> MRLRSPYWLFVVLILALAGLQYRLWVGDGSLAQVRDLQKQIADQHGENERLLERNRILEAEVAELKKGTETVEERARHELGMVKDGETLYQL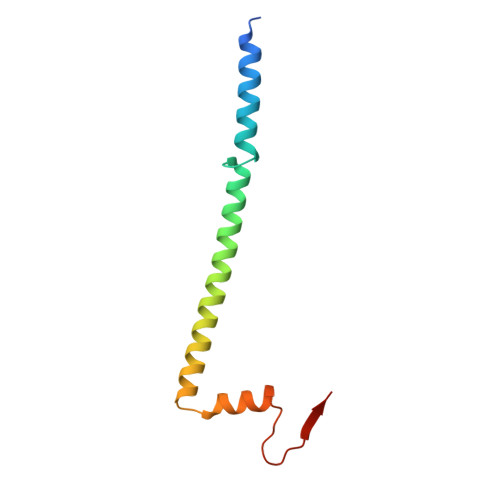AK>MS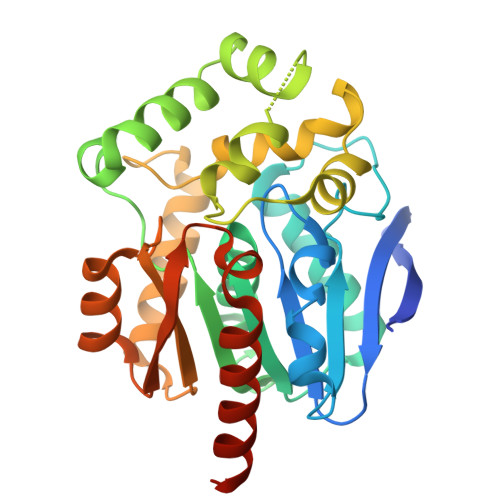TQISAEFPFERRHVEVLGSTMHYVETGEGPPVLFLHGNPTSSYLWRNIIPHVADHGRCIAPDLIGMGQSGKPDIDYRFADHVRYLDAFIDALGLDDVTLVVHDWGSALGFHWARRHPDRVKGIAFMEAIVRPMPSWDDFPPQARELFQALRTPGVGEKMILEQNMFIEKILPGSVLRPLSEEEMDAYRAPFPTPESRKPVLQWPRELPIDGEPADVVAIVEAYAEWLATSDVPKLLFYAEPGALISPEQVEWCRENLPNLEVVHVGPGLHFLQEDQPDAIGQAIADWLQRLASRSSHHHHHH[2x]>MAPAEILNGKEISAQIRARLKNQVTQLKEQVPGFTPRLAILQVGNRDDSNLYINVKLKAAEEIGIKATHIKLPRTTTESEVMKYITSLNEDSTVHGFLVQLPLDSENSINTEEVINAIAPEKDVDGLTSINAGRLARGDLNDCFIPCTPKGCLELIKETGVPIAGRHAVVVGRSKIVGAPMHDLLLWNNATVTTCHSKTAHLDEEVNKGDILVVATGQPEMVKGEWIKPGAIVIDCGINYVPDDKKPNGRKVVGDVAYDEAKERASFI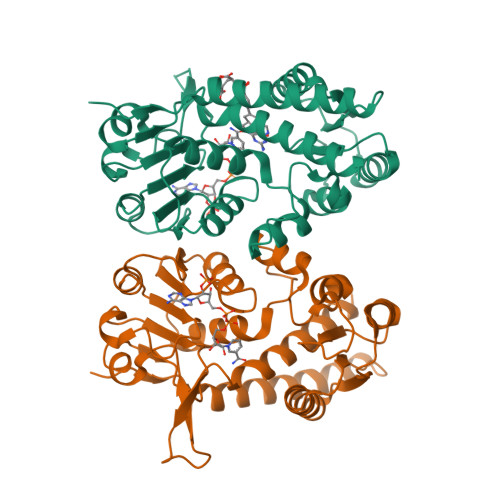TPVPGGVGPMTVAMLMQSTVESAKRFLEKFKPGKWMIQ[2x]> MCLLLFICLYFARGIYCLK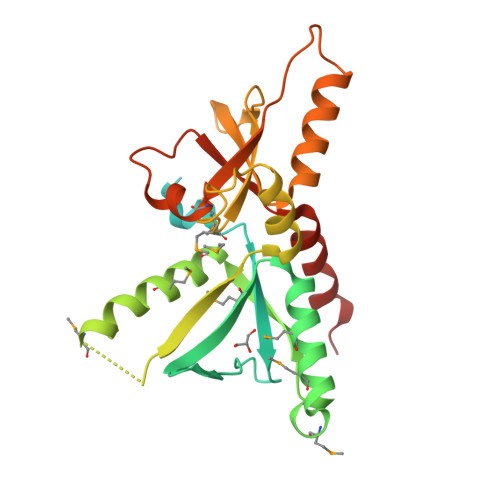TLNGLSRDINNSIYLRNNVHKKKRLVDCNLCMLKHKFRLSFWKKRYDERPIEEKLEVIPVFLITNYNSSPYIFQENEKQVCYMFLCPYDAENMLNDMIKYNGMKYNGNIKIHNITMKKAYELMKEFLQLEKMEVNKEDSKKKQNIYWKLISSKRQLQNALYYLSFTKKSELMYPVFYAENLYIQKDGSNIIPLFFDLEDLKEAIEEQKNKALSKVDYKIKVLNMVDLIFTEDHKKFGFVPSTQSVKYLDKLNIGTKKTYF>[2x]MDLSAASHRIPLSDGNSIPIIGLGTYSEPKSTPKGACATSVKVAIDTGYRHIDGAYIYQNEHEVGEAIREKIAEGKVRREDIFYCGKLWATNHVPEMVRPTLERTLRVLQLDYVDLYIIEVPMAFK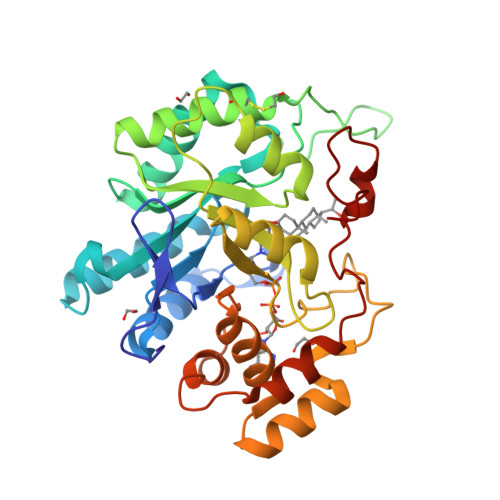PGDEIYPRDENGKWLYHKSNLCATWEAMEACKDAGLVKSLGVSNFNRRQLELILNKPGLKHKPVSNQVECHPYFTQPKLLKFCQQHDIVITAYSPLGTSRNPIWVNVSSPPLLKDALLNSLGKRYNKTAAQIVLRFNIQRGVVVIPKSFNLERIKENFQIFDFSLTEEEMKDIEALNKNVRFVELLMWRDHPEYPFHDEY> MAKKTSGRGKLPPGPTPLPVIGNILQIGIKDISKSLTNLSKVYGPVFTLYFGLKPIVVLHGYEAVKEALIDLGEEFSGRGIFPLAERANRGFGIVFSNGKKWKE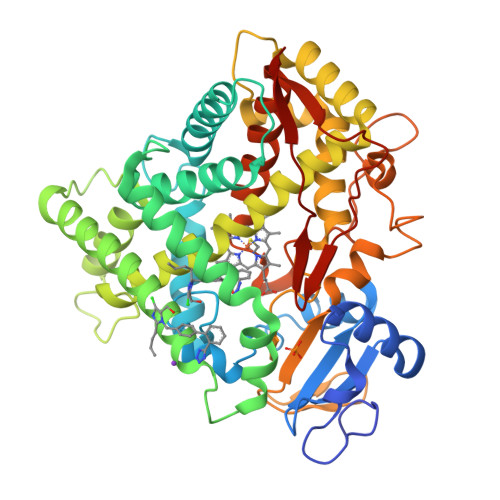IRRFSLMTLRNFGMGKRSIEDRVQEEAHCLVEELRKTKASPCDPTFILGCAPCNVICSIIFHKRFDYKDQQFLNLMEKLNENIKILSSPWIQICNNFSPIIDYFPGTHNKLLKNVAFMKSYILEKVKEHQESMDMNNPQDFIDCFLMKMEKEKHNQPSEFTIESLENTAVDLFGAGTETTSTTLRYALLLLLKHPEVTAKVQEEIERVIGRNRSPCMQDRSHMPYTDAVVHEVQRYIDLLPTSLPHAVTCDIKFRNYLIPKGTTILISLTSVLHDNKEFPNPEMFDPHHFLDEGGNFKKSKYFMPFSAGKRICVGEALAGMELFLFLTSILQNFNLKSLVDPKNLDTTPVVNGFASVPPFYQLCFIPIHHHH>GLPLDERAFEKTLTPIIQEYFEHGDTNEVAEMLRDLNLGEMKSGVPVLAVSLALEGKASHREMTSKLLSDLCGTVMSTTDVEKSFDKLLKDLPELALDTPRAPQLVGQFIARAVGDGILCNTYIDSYKGTVDCVQARAALDKATVLLSMSKGGKRKDS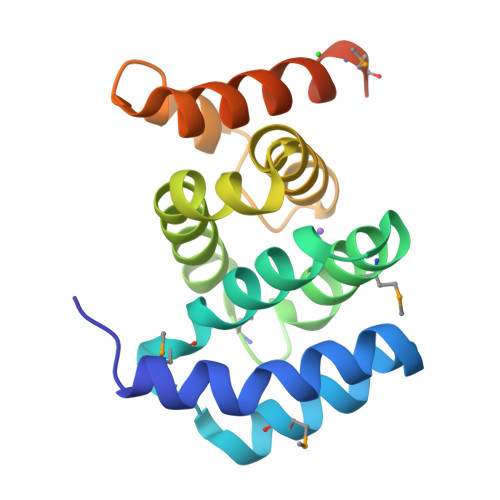VWGSGGG[2x]> DMRPE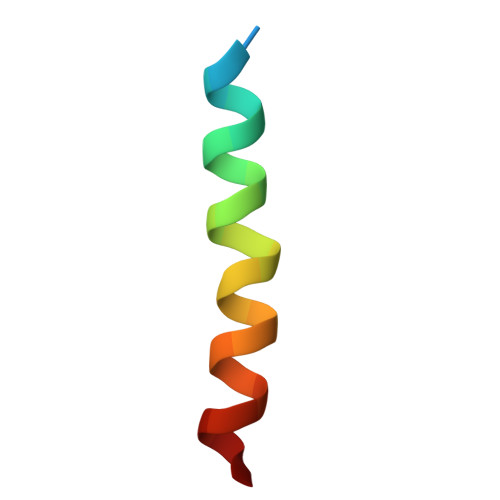IWIAQEFRRIGDEFNAYYARR> DPHMAMEMRLPVARKPLSERLGRDTKKHLVVPGDTITTDTGFMRGHGTYMGEEK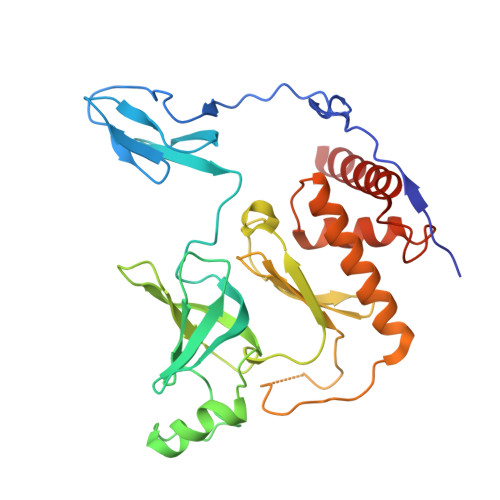LIASVAGSVERVNKLICVKALKTRYIGEVGDIVVGRITEVQQKRWKVETNSRLDSVLLLSSMNLPGGELRRRSAEDELAMRGFLQEGDLISAEVQAVFSDGAVSLHTRSLKYGKLGQGVLVQVSPSLVKRQKTHFHDLPCGASVILGNNGFIWIYPTPEHKEEEAGGFIANLEPVSLADREVISRLRNCIISLVTQRMMLYDTSILYCYEASLPHQIKDILKPEIMEEIVMETRQRLLEQEG>MPNTAMKKKVLLMGKSGSGKTSMRSIIFANYIARDTRRLGATIDVEHSHVRFLGNLVLNLWDCGGLDTFMENYFTSQRDNIFRNVEVLIYVFDVESRELEKDMHYYQSCLEAILQNSPDAKIFCLVHKMDLVQEDQRDLIFKEREEDLRRLSRPLECACFRTSIWDETLYKAWSSIVYQLIPNVQQLEMNLRNFAQIIEADEVLLFERATFLVISHYQCKEQRDVHRFEKISNIIKQFKLSCSKLAASFQSMEVRNSNFAAFIDIFTSNTYVMVVMSDPSIPSAATLINIRNARKHFEKLERVDGPKHSLLMR[2x];>[2x]MSLQYGAEETPLAGSYGAADSFPKDFGYGVEEEEEEAAAAGGGVGAGAGGGCGPGGADSSKPRILLMGLRRSGKSSIQKVVFHKMSPNENLFLESTNKIYKDDISNSSFVNFQIWDFPGQMDFFDPTFDYEMIFRGTGALIYVIDAQDDYMEALTRLHITVSKAYKVNPDMNFEVFIHKVDGLSDDHKIETQRDIHQRANDDLADAGLEKLHLSFYLTSIYDHSIFEAFSKVVQKLIPQLPTLE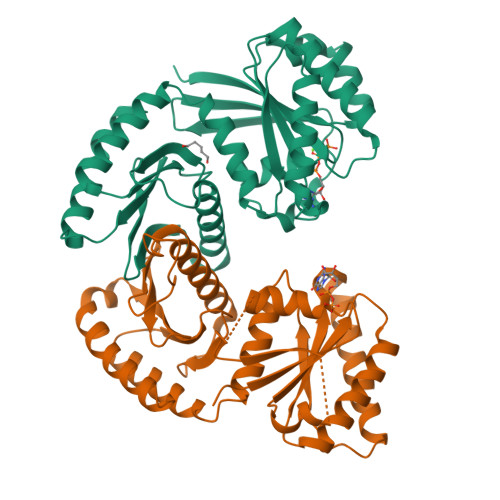NLLNIFISNSGIEKAFLFDVVSKIYIATDSSPVDMQSYELCCDMIDVVIDVSCIYGLKEDGSGSAYDKESMAIIKLNNTTVLYLKEVTKFLALVCILREESFERKGLIDYNFHCFRKAIHEVFEVGVTSHRSCGHQTSASSLKALTHNGTPRNAI> APLGSTYIFSKGGGQITYKWPPNDRPSTRADRLAIGFSTVQKEAVLVRVDSSSGLG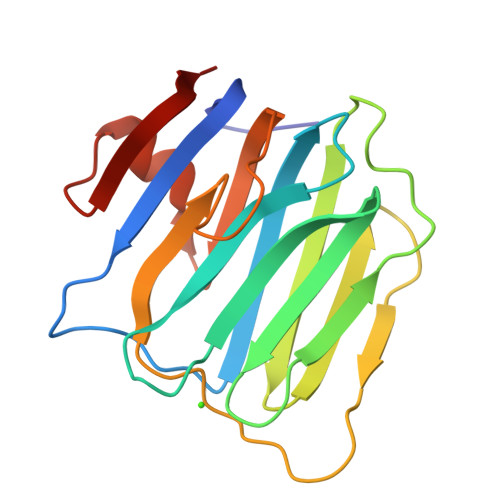DYLELHIHQGKIGVKFNVGTDDIAIEESNAIINDGKYHVVRFTRSGGNATLQVDSWPVIERYPAGRQLTIFNSQATIIIGGKEQGQPFQGQLSGLYYNGLKVLNMAAENDANIAIVGNVRLV> MTPPLATTIDRLRDYLDRVGFQQIYKYIVAVNHYAVTPALITRNTAASVHHFFDSRLGGRAEFALLQCLMTGRPAEHAALPDKDRALADALVTAGLLRASPDGREVSGADRQLISAFGVDLLIDRRIHFGGEVHEVYIGPDSYWMLYYINASGIARTHRAVDLCTGSGIAALYLSLFTDHVLATDIGDVPLALVEINRRLNRRDAGTMEIRRENLNDTLDGRERFDLLTCNPPF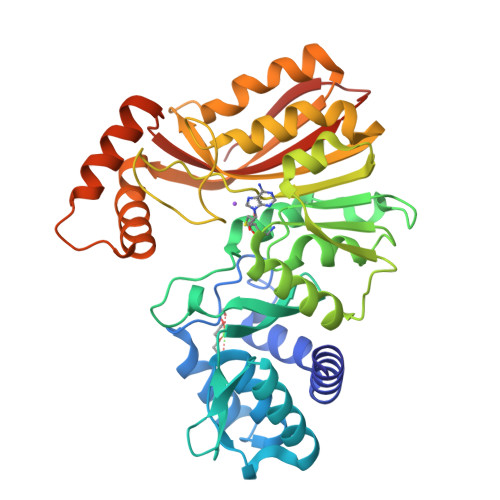VAFPPGYSGTLYSQGTGVDGLGYMRDIVGRLPEVLNPGGSAYLVADLCGDAHGPHFLGELESMVTGHGMRIEAFIDHVLPASAQVGPISDFLRHAAGLPADTDIAADVQAFQRETLRADYYYLTTIRLQTAAQNPGLRMLRRDPLPGAGT>[4x]SNAMNTVCTACMATNRLPEERIDDGAKCGRCGHSLFDGEVINATAETLDKLLQDDLPMVIDFWAPWCGPCRSFAPIFAE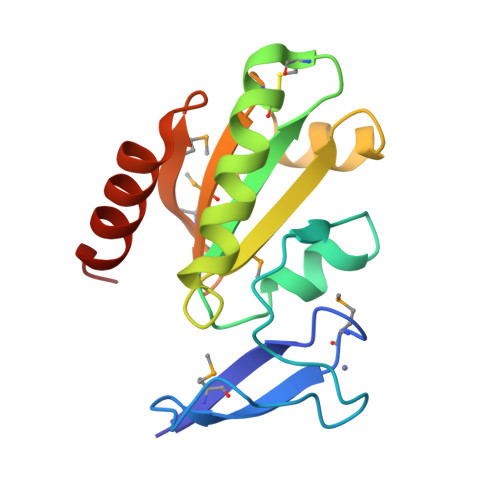TAAERAGKVRFVKVNTEAEPALSTRFRIRSIPTIMLYRNGKMIDMLNGAVPKAPFDNWLDEQLSRDPNS> GKKCYKLENEKLFEEFLELCKMQTADHPEVVPFLYNRQQRAHSLFLASAEFCNILSRVLSRAR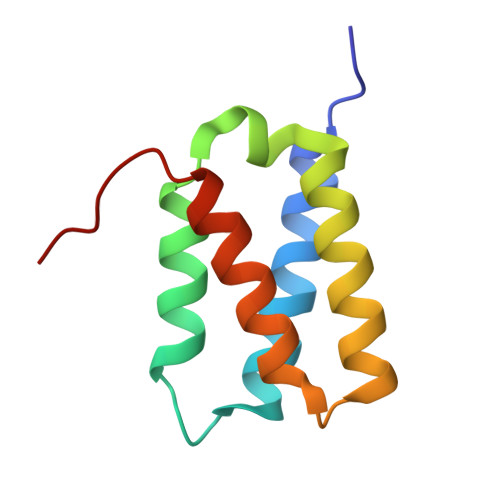SRPAKLYVYINELCTVLKAHSAKKKLN>[2x]MAEDPDPTEYLYISMEQKRKDQTKPYDGKKMVWVADEKEGYLLGLIKSTQGDICTVDIEGQESRQVKKDLLQQVNPPKYEKCEDMSNLTYLNDASVLHNLKQRYYANLIYTYSGLFCVAINPYKRFPIYTNRTVQIYKGRRRTEVPPHLFAISDGAYSAMLANRENQSMLITGESGAGKTENTKKVIAYYANVGAATPKPGKEAPTKEKKATLEDQVVQTNPVLEAFGNAKTVRNDNSSRFGKFIRIHFGPMGKLAGADIETYLLEKARVISQQTLERSYHIFYQLMSGGIENLKADLLLSDDIYDYHFVSQGKIEIPGVDDAEELRLTDTAFDILGFSHEYKTDVYKITASCMHLGEMKFKQRPREEQAEADGTEEGERVAHLLGVNAADLYKNLVKPKIKVGNEMVTQGRNATQVSYSVGGLAKAMFDRTFKWLVKRLNETLDTKQKRQYFIGVLDIAGFEIFDYNGFEQLCINFTNEKLQQFFNHHMFVLEQEEYKREGIDWVFIDFGLDLAACIELIEKPMGILSILEEESMFPKATDKSFQDKLNANHLGKSPNFVKPKPPKPGQQEAHFSIAHYAGTVPYNITGWLEKNKDPVNDTVVDQFKKGSNKLVQEIFEDHPGLGAEEKGGGGKGGGGRKKGASFQTVSALYREQLNRLMASLHSTQPHFVRCIIPNELKQPGVIDSGLVMHQLTCNGVLEGIRICRKGFPNRMVYPDFKQRYTILAASAVPKGFVDAKKVTEAVLGAIQLDANDYRLGNTKVFFRAGVLGRLEEMRDDRLGKIVTWLQAWIRWYLSKKEFKKLQEQRVALLVIQRNLRKFLTLRNWLWYKLYIKVKPLLTMAKVEDELKALEEKLKKALESLEKEEKVRKDIEVQNVKLLQEKNDLFLQLESERSGAGDVEERLTKAISMKNDLEGQVQELQERLSREEDAHSNLSSVRKKLDGEISNLKKEIEDLQLVIQKTEQDKAAKDHQIRNLNDEIAHQDELINKLNREKKQMQEMGQKTGEDLQATEDKLNHMNKVKAKLEQTLDELEDSLEREKKLRGDVEKTKRKVEGDLKLAQEAVADLEKNKKELEQALQRKEKEMASLSAKLEDEQGLVAKLQKQIKELQARIEELEEELEAERQARAKAEKQRADLAREIEELSERLEEAGGATSAQVELNKRREAEMAKLRRDLEESNIQHEQTLANLRKKHNDVVAELSEQIDQLNKHKARLEKEKAQMKGELDDVRSSVDHVNKEKANAEKQAKQLEMQLTELQGKMDEAHRSLGDFDAAKKRLTVENTELTRQLEDAESQVSQLSKLKTSLQTQLEDTKRMADEESRERATAMGKFRSVEHDLDSLREQIDEEQEGKADLQRQLSKANAEVQLWRSKYESEGLARLEELEESKRKLDAKLQEAMETIDQLNSKTSGLEKTKSRLQGELEDMTIEVEKANALASAMEKKQKSFDRIISEWKQKVDDLALELDASQKECRNYSTEVFKLRSQYEESQEHYESVKRENKNLQDEIKDLVDQLGEGGRSVHELEKARKRLELEKEELQAALEEAEAALEQEENKVLRAQLELSQVRQEIDRRLQEKEEEFENTRKNHQRAIDSMQASLEAEAKGKAEALRMKKKLESDINELEIALDHSNKANAEAQKNIKKYQIQLKETQQALEEEQRARDEVREQYAMSERRCNAMHGELEESRQLLEQADRARRAADSELAELHENVNELSAQNSSLSMAKRKLEGEMQALHADLDEMLNEAKSSEEKAKKAMVDAARLADELRAEQEHAQQQEKMRKAMEGQIKELQVRLDEAEAAALKGGKKIIQKLEQKVRELETELDNEQRRHSEAAKNVRRSERRVKELQFQAEEDRKNQERMQDLVDKLQQKIKTYKRQIEEAEEIAALNLAKFRKVQQELEDAEERADMAENVAAKLRAKNRSSASVGRAMSPIPMGKPGRPKSKIDEE;>[2x]MADLKAAEVEKAREHFEIYDWEGEGKIDARDLGDLLRSLDCKPTLAMVKKNGGSDKRGEKKLTLEEFLPIFSQIKKEKEVGTLEDFMEGLKVYDKAENGTMLAAELAHVLLSLGERLTDIECEEIMRVCDEDDDGFLKYEPFVKTIIAGPFPDEGK;>[2x]MGDEEKKEKKKKSKKKSEEEGGDAAPAPPPPKPPSQKRRAQRSGSNVFAMFTQHQVQEFKEAFQLIDQDKDGFISKNDIRATFDSLGRLCTEQELDSMVAEAPGPINFTMFLTIFGDRIAGTDEEDVIVNAFNLFDEGEGKCKEETLKRSLTTWGEKFSQDEVEEALSEAPIDGNGLIDIKKFAQILTKGAEEEGA

More recently, with improvements in EM techniques, higher resolution studies have homed in on one particular kind of structure for the myosin head arrays in relaxed muscles. This configuration is the so-called interacting head motif (IHM) first observed in 2D crystals of isolated myosin heads from vertebrate smooth muscle. Studies of isolated myosin filaments by electron microscopy (EM) have been carried out for many years and 3D reconstructions and other kinds of analysis have revealed the rotational symmetry of these myosin filaments: 3-fold for vertebrates, 4-fold for insect flight muscle.

Here we deal with the myosin filament structures in vertebrate striated (i.e., fish skeletal and human cardiac) muscles and insect flight (Lethocerus) muscles. We have shown in our analysis that the interacting head motif structures for the myosin filaments in a vertebrate muscle (bony fish) and an insect flight muscle (Lethocerus) do not explain the X-ray diffraction observations previously recorded from these same muscles in the resting state as well as our original fitted structures. Turning now to insect flight muscle, the same story appears to hold true there. The compact interacting head motif structure is not the best fit to the observed X-ray diffraction data. The preferred structure that better fits the layer-line pattern has one of the bridges extending radially outwards towards actin, with the other head closer to the backbone in the same position as the outer head in the IHM structure in Figure 12a. The blocked head, on the other hand, would then stay in almost the same place in both the super-relaxed state and the “activated” relaxed state. In either case, activation puts one of each head pair very close to an actin filament. Using further analysis of the low-angle X-ray diffraction data from bony fish muscle and insect flight muscle it has been demonstrated that the normal resting state of in both intact muscles in the published X-ray diffraction experiments is probably not the IHM, super-relaxed state that has been seen in 3D single particle reconstructions from electron microscopy.>MGAIESRKLLASETPVGQFIPYSHHVTDTIISTKNAEYLSVWKIDGRSHQSASEADVFQWIRELNNTLRGISSANLSLWTHIVRRRVYEYPDAEFDNVFCRQLDEKYRESFTGYNLMVNDLYLTVVYRPVSDKVLSFFAKRERETPDQKKHRQESCIKALEDINRTLGQSFKRYGAELLSVYEKGGHAFSAPLEFLARLVNGEHIPMPICRDRFSDYMAVNRPMFSKWGEVGELRSLTGLRRFGMLEIREYDDATEPGQLNVLLESDYEFVLTHSFSVLSRPAAKEYLQRHQKNLIDARDVATDQIEEIDEALNQLISGHFVMGEHHCTLTVYGETVQQVRDNLAHASAAMLDVAVLPKPVDLALEAGYWAQLPANWQWRPRPAPITSLNFLSFSPFHNFMSGKPTGNPWGPAVTILKTVSGTPLYFNFHASKEEEDATDKRLLGNTMLIGQSSSGKTVLLGFLLAQAQKFKPTIVAFDKDRGMEISIRAMGGRYLPLKTGEPSGFNPFQLPPTHANLIFLKQFVKKLAAAGGEVTHRDEEEIDQAITAMMSDSIDKSLRRLSLLLQFLPNPRSDDMDARPTVHARLVKWCEGGDYGWLFDNPTDALDLSTHQIYGFDITEFLDNPEARTPVMMYLLYRTESMIDGRRFMYVFDEFWKPLQDEYFEDLAKNKQKTIRKQNGIFVFATQEPSDALESNIAKTLIQQCATYIFLANPKADYEDYTQGFKLTDSEFELVRGLGEFSRRFLIKQGDQSALAEMNLGKFRTIVDGETVERDFDDELLVLSGTPDNAEIAESIIAEVGDDPAVWLPIFLDRVKAERSDV[2x];> MKPPQQQHEAFPLFKGATRLPTIWGVPMIPLMAM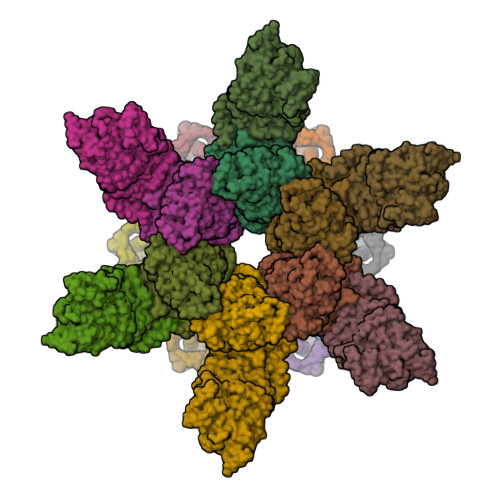VMGVAVIALTVSIWWWALVPPLWFIMAQITKNDDKAFRIWWLWIDTKFRNRNKGFWGASSYSPANYRKRR;>[3x]MSKKQPKPVKAEQLKSYYEESRGLERDLIGEFVKSRKTAWRVATASGLFGLLGMVCGIVGFSQPAPAPLVLRVDNATGAVDVVTTLREHESSYGEVVDTYWLNQYVLNREAYDYNTIQMNYDTTALLSAPAVQQDYYKLFDGSNARDRVLGNKARITVRVRSIQPNGRGQATVRFTTQQHNSNGTVEAPQHQIATIGYTYIGAPMRSSDRLLNPLGFQVTSYRADPEILNN>MLDPKLVRTQPQEVAARLATRGFQLDVARIEALEEQRKSVQTRTEQLQAERNARSKAIGQAKQRGEDIAPLLADVDRMGSELEEGKRQLDAIQGELDAMLLGIPNLPHESVPVGADEDANVEVRRWGTPKTFDFEVKDHVALGERHGWLDFETAAKLSGARFALMRGPIARLHRALAQFMINLHTAEHGYEEAYTPYLVQ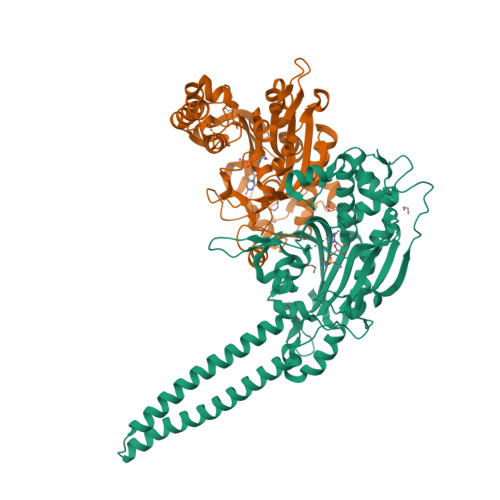APALQGTGQLPKFEEDLFKIGRDGEADLYLIPTAEVSLTNIVSGQILDAKQLPLKFVAHTPCFRSEAGASGRDTRGMIRQHQFDKVEMVQIVDPATSYEALEGLTANAERVLQLLELPYRVLALCTGDMGFGSTKTYDLEVWVPSQDKYREISSCSNCGDFQARRMQARYRNPETGKPELVHTLNGSGLAVGRTLVAVLENYQQADGSIRVPEVLKPYMAGIEVIG[2x]> HHHHHHHMMDFGALPPEINSARMYAGAGAGPMMAAGAAWNGLAAELGTTAASYESVITRLTTESWMGPASMAMVAAAQPYLAWLTYTAEAAAHAGSQAMASAAAYEAAYAMTVPPEVVAANRALLAALVATNVLGINTPAIMATEALYAEMWAQDALAMYGYAAASGAAGMLQPLSPPSQTTNP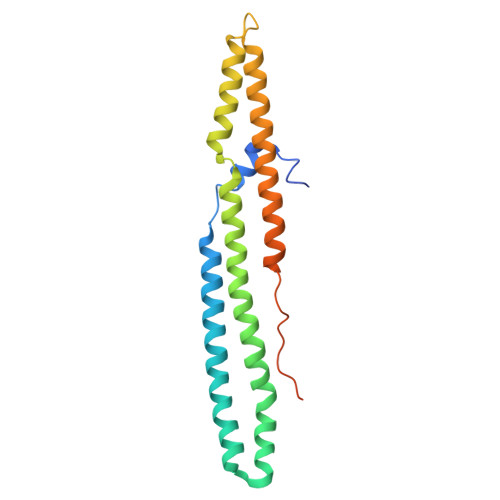GGLAAQSAAVGSAAATAA>[2x]GTQNDRMPGPELSGWISEQLMTGRIPVSDIFCDIENNPGLCYASQMQGIVRQRVIPVYQVNNLEEICQLIIQAFEAGVDFQESADSFLLMLCLHHAYQGDYKLFLESGAVKYLEGHGFRFEVKKRDGVKRLEELLPAVSSGKNIKRTLAAMPEEETTEANAGQFLSFASLF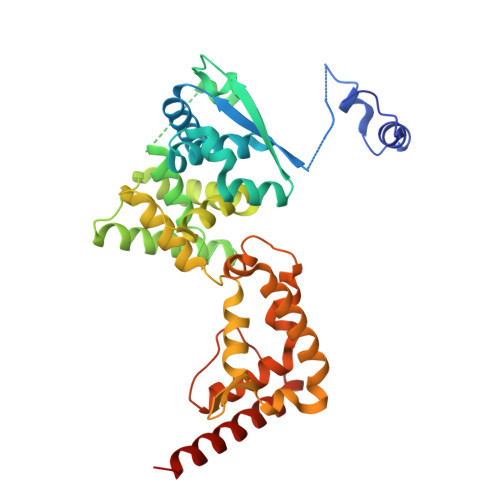LPKLVVGEKACLEKVQRQIQVHAEQGLIQYPTAWQSVGHMMVIFRLMRTNFLIKFLLIHQGMHMVAGHDANDAVISNSVAQARFSGLLIVKTVLDHILQKTERGVRLHPLARTAKVKNEVNSFKAALSSLAKHGEYAPFARLLNLSGVNNLEHGLFPQLSAIALGVATAHGSTLAGVNVGEQYQQLREAATEAEKQLQQYAESRELDHLG> GSTSLGRPEEEEDELAHRCSSFMAPPVTDLGELRRRPGDMKTKMELLILETQAQVCQALAQVDGGANFSVDRWERKEGGGGISCVLQDGCVFEKAGVSISVVHGNLSEEAAKQMRSRGKVLKTKDGKLPFCAMGVSSVIHPKNPHAPTIHFNYRYFEVEEADGNKQWWFGGGCDLTPTYLNQEDAVHFHRTLKEACDQHGPDLYPKFKKWCDDYFFIAHRGERRGIGGIF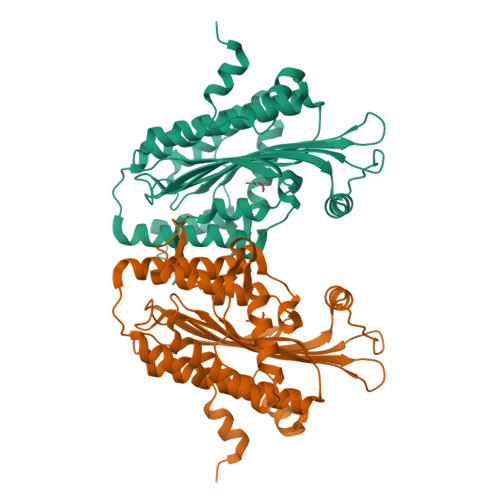FDDLDSPSKEEVFRFVQSCARAVVPSYIPLVKKHCDDSFTPQEKLWQQLRRGRYVEFNLLYDRGTKFGLFTPGSRIESILMSLPLTARWEYMHSPSENSKEAEILEVLRHPRDWVR>[2x]MSRGALIVFEGLDKSGKTTQCMNIMESIPANTIKYLNFPQRSTVTGKMIDDYLTRKKTYNDHIVNLLFCANRWE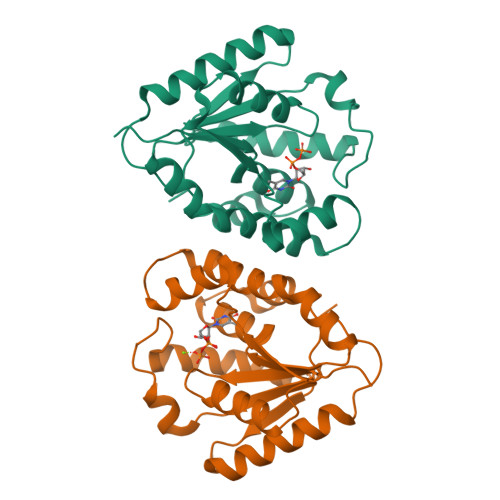FASFIQEQLEQGITLIVDRYAFSGVAYAAAKGASMTLSKSYESGLPKPDLVIFLESGSKEINRNVGEEIYEDVTFQQKVLQEYKKMIEEGDIHWQIISSEFEEDVKKELIKNIVIEAIHTVTGPVGQLWM> MHHHHHHGSGDKEKKQITTSPITVRKNKKDEERRESRIQSYSPQAFKFFMEQHVENVLKSHQQ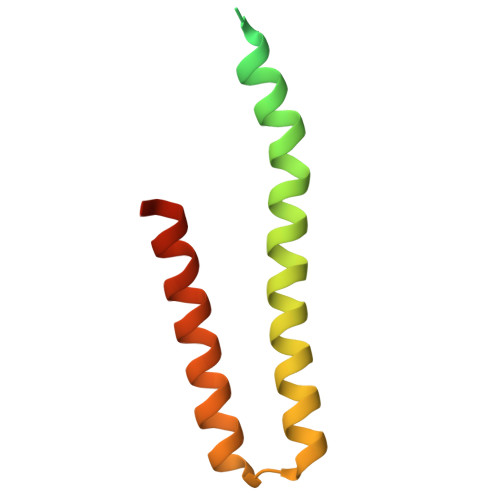RLHRKKQLENEMMRVGLSQDAQDQMRKMLCQKESNYIRLKRAKMDKSM>GPGMAVKHLFVLKFKDEITEAQKEEFFKTYVNLVNIIPAMKDVYWGKDVTQKNKEEGYTHIVEVTFESVETIQDYIIHPAHVGFGDVYRSFWEKLLIFDYTPRK[4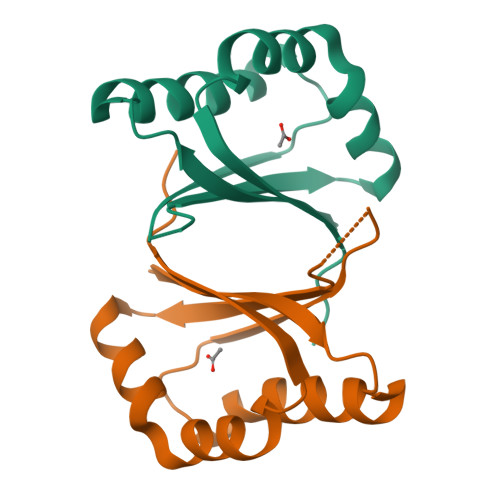x]> EIVEPEFPHNAIEPCVICQTRPKNGCIVHGKTGHLMACFTCAKK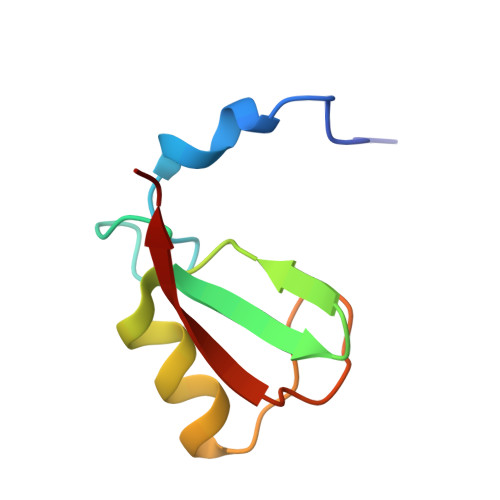LKKRNKPCPVCRQPIQMIVLTYFP>[2x]GHMTKLNQESTAPKVLFTGVVDARGERAVLALGGSLAGSAAEASHLVTDRIRRTVKFLCALGRGIPILSLD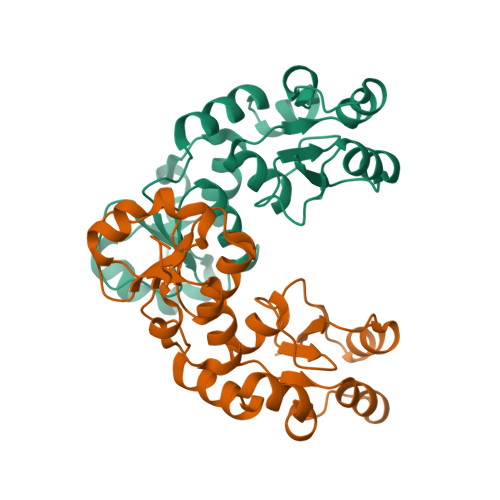WLHQSRKAGFFLPPDEYVVTDPEQEKNFGFSLQDALSRARERRLLEGYEIYVTPGVQPPPPQMGEIISCCGGTYLPSMPRSYKPQRVVITCPQDFPHCSIPLRVGLPLLSPEFLLTGVLKQEAKPEAFVLSPLEMSST>GAMAMANSERTFIAIKPDGVQRGLVGEIIKRFEQKGFRLVGLKFLQASEDLLKEHYTDLKDRPFFTGLVKYMHSGPVVAMVWEGLNVVKTGRVMLGETNPADSKPGTIRGDFCIQVGRNIIHGSDSVKSAEKEISLWFQPEELVEYKSCAQNWIYE[6x]

In mammals, the most abundant and best-studied NDPKs are NME1 and NME2 (hereafter abbreviated NME1/2), which are closely related isoforms (88% sequence identity) with similar functional attributes and localization in the cytosol and nucleus. NME1/2 are hexameric enzymes that catalyze the reaction XTP + YDP ⇆ XDP + YTP by first transferring the γ-phosphoryl group from XTP (usually ATP) to residue His118, and then from the phosphohistidine to YDP, where Y is any of the four common (deoxy)nucleosides. Briefly, each NME1 subunit within the D3-symmetric hexamer comprises an antiparallel four-stranded β sheet flanked on either side by a layer of helices. In this study, we showed that NME1 binds AcCoA and CoA with similar affinity via a binding mode distinct from that of canonical ADP and ATP substrates and critically dependent on the CoA 3′ phosphate group.

Efforts to cocrystallize murine NME1 with the ligands led to high-resolution (1.96 and 2.2 Å, respectively) crystal structures of NME1 bound to SucCoA and ADP, and a somewhat lower (2.6 Å)–resolution structure bound to CoA. CoA and SucCoA bind to this site via their common nucleotide moiety, the only part of these ligands specifically recognized by NME1. Unexpectedly, NME1 recognizes ADP and CoA via completely distinct binding modes. NME1 recognizes the 3′ phosphate group that distinguishes CoA from ADP with high specificity via five direct and two water-mediated H bonds. The CoA 3′ phosphate group forms direct H bonds with Lys12, Tyr52, Asn115, and His118 as well as water-mediated H bonds with Arg88, Arg105, and the Gly119 backbone. First, as in the ADP complex, the adenine base of CoA is sandwiched between hydrophobic residues from the Kpn loop and αA-α2 helical hairpin but is rotated by ~40° in the plane of the base to compensate for the shifted ribose ring and maintain a stacking interaction with residue Phe60. Compared to ADP, the α and β phosphates of CoA are displaced upward and are solvent accessible, pointing out of the pocket to direct the CoA pantetheine end away from the protein surface. Arg58 forms a salt bridge with the CoA α phosphate in a subset of NME1 subunits. The recorded profiles revealed that the melting temperature of NME1 (Tm = 60°C) was enhanced similarly by each of the tested ligands (ΔTm ≈ 3.7°C), confirming that AcCoA and SucCoA bind NME1 with similar affinity to CoA. Since the latter affinity has not been previously quantified, we analyzed the NME1:CoA interaction by isothermal titration calorimetry (ITC).>MSVHATDAKPPGPSPADQLLDGLNPQQRQAVVHEGSPLLIVAGAGSGKTAVLTRRIAYLMAARGVGVGQILAITFTNKAAAEMRERVVGLVGEKARYMWVSTFHSTCVRILRNQAALIEGLNSNFSIYDADDSRRLLQMVGRDLGLDIKRYSPRLLANAISNLKNELIDPHQALAGLTEDSDDLARAVASVYDEYQRRLRAANALDFDDLIGETVAVLQAFPQIAQYYRRRFRHVLVDEYQDTNHAQYVLVRELVGRDSNDGIPPGELCVVGDADQSIYAFRGATIRNIEDFERDYPDTRTILLEQNYRSTQNILSAANSVIARNAGRREKRLWTDAGAGELIVGYVADNEHDEARFVAEEIDALAEGSEITYNDVAVFYRTNNSSRSLEEVLIRAGIPYKVVGGVRFYERKEIRDIVAYLRVLDNPGDAVSLRRILNTPRRGIGDRAEACVAVYAENTGVGFGDALVAAAQGKVPMLNTRAEKAIAGFVEMFDELRGRLDDDLGELVEAVLERTGYRRELEASTDPQELARLDNLNELVSVAHEFSTDRENAAALGPDDEDVPDTGVLADFLERVSLVADADEIP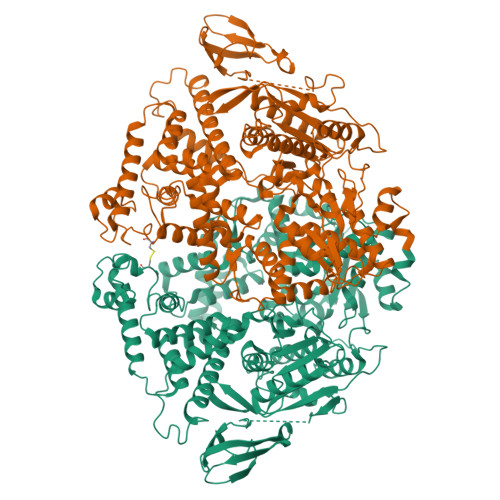EHGAGVVTLMTLHTAKGLEFPVVFVTGWEDGMFPHMRALDNPTELSEERRLAYVGITRARQRLYVSRAIVRSSWGQPMLNPESRFLREIPQELIDWRRTAPKPSFSAPVSGAGRFGSARPSPTRSGASRRPLLVLQVGDRVTHDKYGLGRVEEVSGVGESAMSLIDFGSSGRVKLMHNHAPVTKL[2x]>[12x]IELPDAISDGEVRKLVENEFWPEFVRRREKLDRIAQWARGEQPDYLIQNANREKRALLKLAKTPWLGLVVTHFTQALFVDGYRAEGSKENAKGPWQTWNANKMQSKQIAIHRAALTYGYSYARVLPGVALDGANQAEIHGVSPRRLLALYEDQINDEYPKYALELANNGKTVRLYTDTDYYELRMPSPGNFPNEQVIKKVHHGVGVCPFVRYVNMMDLDGFTMGEVEYLVPVASKIDKTDYDRLLAQHYNSWKVKVATGIDDLSEDATPEEQQRAKLILAQDDILMHGNHEAKFYTLPETSLDGFIAAHTQDVEILANNAQVPVWILNGQLANLSADALTAATKGTIQKLYERQVTFGAAHNQVLRLAAHVEGDTEGARDFTASVSWQDTSVRSLAQAVDAYGKAATMLGMPKEFLWGLIPGITKTDVEAMRQHFNDDDEMTQMLLWWTPNGPGGEFAAE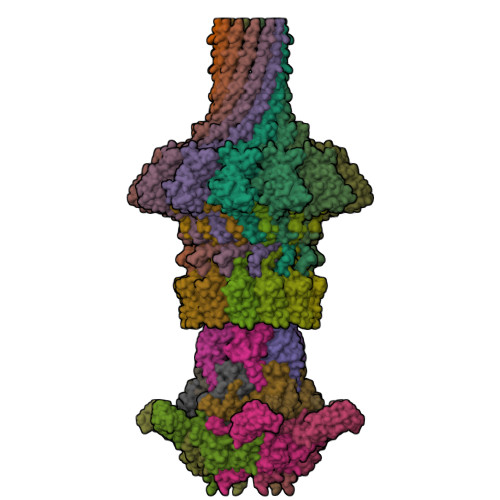IEVDSQTQIIEAQGDVQKDLQDAQAKAQADLAKQNAAAQQRQAVAV;>[6x]MNDETLTVYRGATDNKGNPNKQVHGTVKGVFAWGPGTSTNKFGRDRNFKGESSSLTAELYVKRGADLKARDRIRRANGEEYSVVGHAAWDQGHPFDGFDFGYMVFQVEAVN;>[6x]TDFYTIKDAQADLAIAPLNLTVLLAPYSTTPATTLESPTDGSLAIPPGYKSVGHFEKQAGLTLGNEFDSKDIEAYGEPEPIRTIINKRTTTFDFAMYQNQRNVLELIWTQDFSNIQPSEFGGIVLEAPKVPKNIYYRAILVGMDDRNDRPIWLYWLMPKVKLDKLDNQTLNDDNVIEYKPTLKAFRDDVVGYSVAQGFAGPGWRDLVATAGFGEALTALTITPGSPTVTVATGASHTAQLLVEGDNGINYTPDVVFTSSAPDKASVSAAGLVTGVAAGSATITATKGALTATATVTVTA;>AGLATIDELQTLMSTVFEDDALEQAQLVLDIVSSWARVVSGQMWPDAPANVPDDVRAVVLQASRRELKNPDRVISRQMGPFNVQYSQPPDGFFYPAELAILKRFKRSGGLMTVSTSRGEEGRPWAGKTAYIRYGDGL[12x];>[6x]AVVLPDWYEEAFVNVENLFIDMFTDLLPDYESGCWAPDDWLADEIEVKPTIWFFRLPGGRVDWDGRKDECQLQVMVVTGSRDDSWRLMDFVRAMLLPMQGDKYKMADGYTAQIRCAGEVAGPQLLTPGQRIDTRVVTATFKVSVSMKSAKNYKQKLYELWQALRG> IQINQVR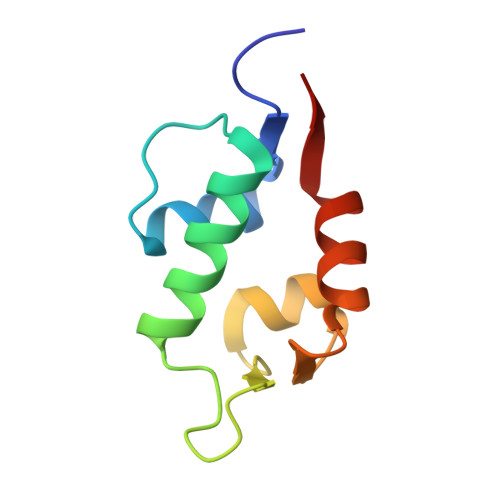PKLPLLKILHAAGAQGEMFTVKEVMHYLGQYIMVKQLYDQQEQHMVYCGGDLLGELLGRQSFSVKDPSPLYDMLRKNLVTLAT>[2x]MELGAGGVVFNAKREVLLLRDRMGFWVFPKGHPEPGESLEEA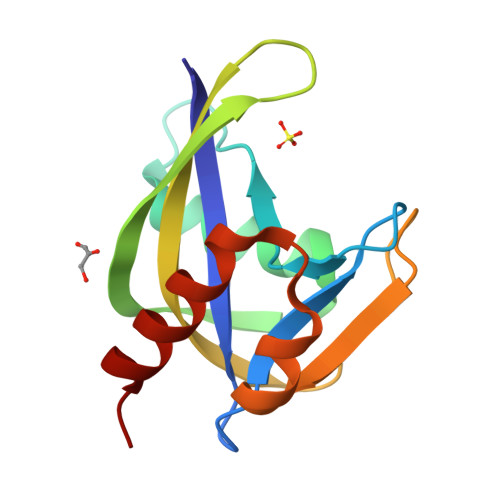AVREVWEETGVRAEVLLPLYPTRYVNPKGVEREVHWFLMRGEGAPRLEEGMTGAGWFSPEEARALLAFPEDLGLLEVALERLPL> GNMSEVINFDQIFEGAIEPGKEPKRLFKEVYEGAITATSYAEILLSRAIEKYGPDHPVGYPDTAYFLPVIRAFSGEEVRTLKDMVPILNRMRAQIKSELTFENARLAGEATWYAAEIIEALRYLKHTPENPIVVPPWTGFIGDPVVRQYGIKMVDWTIPGEAIIIGRAKDSKAAKKIVDDLMGKGLMLFLCDEIIEQLLEENVKLGVDYIAYPLGNFTQVVHAANYALRAGLMFGGIAPGLRDAHRDYQRRRVLAFVLYLGEHDMVKTAAAMGAIFTGFPVITDQ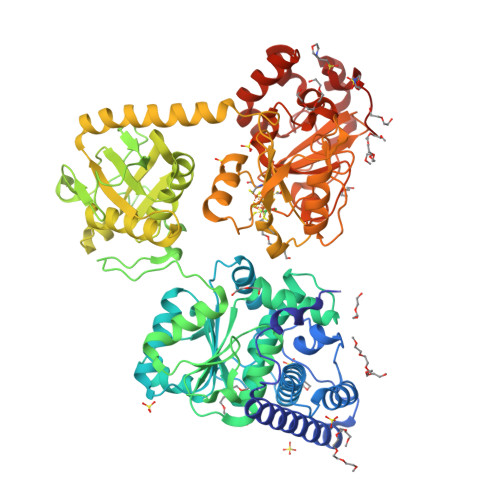PLPEDKQIKDWFISEPDYDKIVQTALEVRGIKITSIDIDLPINFGPAFEGESIRKGDMHVEFGGGKTPSFELVRMVGPDEIEDGKVEVIGPDIDSVEPGGRLPIGIVVDIYGRKMQEDFEPVLERRIHYFTNYGEGFWHTAQRDLTWVRISKEAFAKGARLKHLGQLLYAKFKQEFPSIVDRVQVTIYTDEQKVLELREIARKKYAERDARLRELSDEAVDTYYSCLLCQSFAPTHVCIVSPERVGLCGAISWLDAKAAYEINPNGPNQPIPKEGLIDPVKGQWESFNEYIYKNSQRTIERMNLYTIMEYPMTSCGCFEAIMAYLPELNGFMIVNREHSGMTPIGMTFSTLAGMVGGGTQTPGFMGIGKSYIGSRKFVKADGGLARVVWMPKDLKEQLRSIIEERAEEEGLGRDFIDKIADETVGTTVDEVLPFLEEKGHPALSMEPLL> MTDRPDHIDSRVWELSETQEDWITQVHGHVRRVV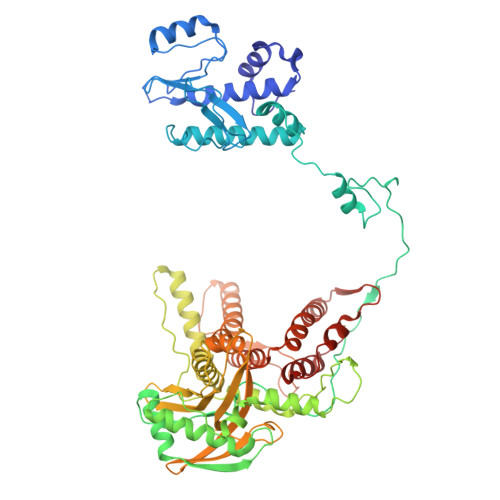ECWKYTICCLISNMHTHRGAPQYDVFKWQDRSTIEWICSKKKVQYPERDTPDLYDNERAVAYKVLLVSDLSDHSPTSGIYHDLAFNLEGEAEESCALVLRGSQLQDIKGFLCRALEWVVSNNLTQEVVETISGEAKLQFSVGTTFRTLLKRDTDWDVIPTPRVEPNVPRIEGRRWTQMKKLPLLKEKEGPPSPWRALLLGADSEYIVCPPGTDQEAISWIHSQSEIECIRESKSTPASVITCLTSSLQSFAEGNPVRSRIHEDIIAFGINKKQEKKQSASSSASGEWKRAEYQVEEMSLPPWVEEEMVLLRSDQEDNWIELEKNAIYTEVDGVAEGLVDKYIEIVGRTKVASVIEKWQIAATRTFSQLHTDRSRITACPIITRDPSGNCQFWGMVLLGPHHVKRDTDNAPLLIAEIMGEDTEEKYPKHSVFSLKVEGKQFLLSLKITSFSRNKLYTFSNIRRVLIQPASIYSQVVLSRAAENNSLNLEVNPEIQLYLEGAQRGMTLYQWVRMILCLEFLMAIYNNPQMEGFLANMRRLHMSRHAMMERRQVFLPFGSRPEDKVNECIINNPIVAYLAKGWNSMPNVYY>MTLPQTMKAAVVHAYGAPLRIEEVKVPLPGPGQVLVKIEASGVCHTDLHAAEGDWPVKPPLPFIPGHEGVGYVAAVGSGVTRVKEGDRVGIPWLYTACGCCEHCLTGWETLCESQQNTGYSVNGGYAEYVLADPNYVGILPKNVEFAEIAPILCAGVTVYKGLKQTNARPGQWVAISGIGGLGHVAVQYARAMGLHVAAIDIDDAKLELARKLGASLTVNARQEDPVEAIQRDIGGAHGVLVTAVSNSAFGQAIGMARRGGTIALVGLPPGDFPTPIFDV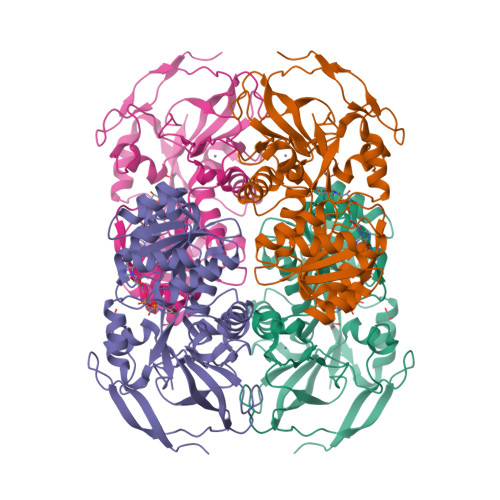VLKGLHIAGSIVGTRADLQEALDFAGEGLVKATIHPGKLDDINQILDQMRAGQIEGRIVLEM[8x]(1R,2R,3R,4R,5R,6S)-2,3,4,5,6-pentahydroxycyclohexyl 2-amino-2-deoxy-alpha-D-glucopyranoside | C12 H23 N O10 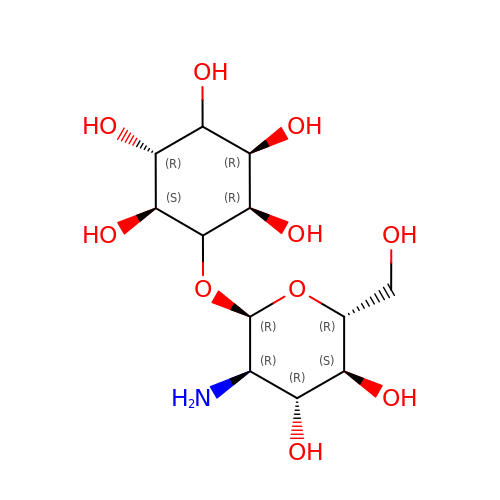| HEPUIGACZYVUCD-YZRQSVRMSA-N4-[4-(6-methoxynaphthalen-2-yl)-1H-imidazol-5-yl]pyridine | 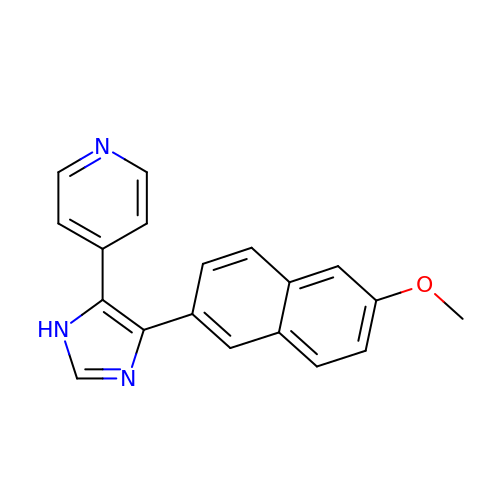C19 H15 N3 O | DXOWEAIMGARAMG-UHFFFAOYSA-N> IPASEQETLVRPKPLLLKLLKSVGAQKDTYTMKEVLFYLGQYIMTKRLYDEKQQHIVYCSNDLLGDLFGVPSFSVKEHRKIYTMIY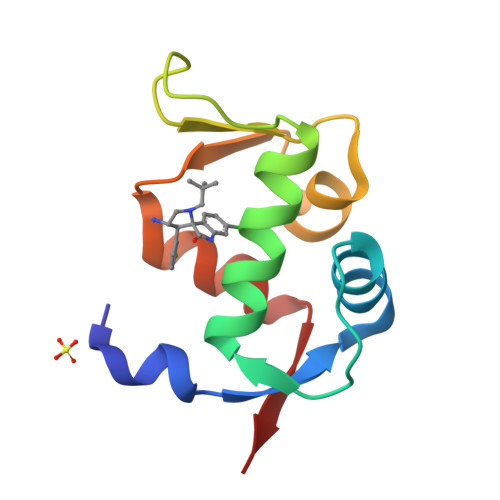RNLVVVN> 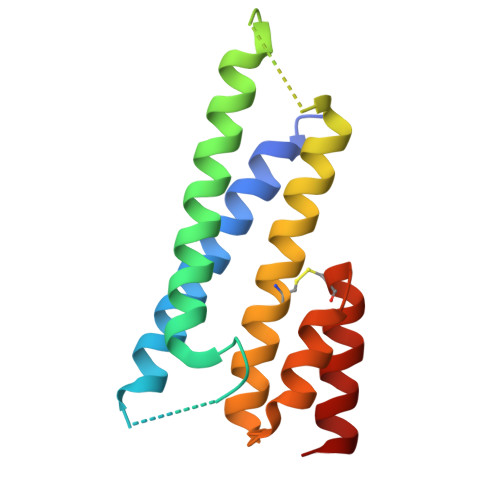GSHMSTEQIQKRTAAIQKRIAAIQKRIYAMTASGGAGAAGAGAGMSIEEITKQIAAIQLRIVGDQVQIAYQTASGAGAGAGGMSTEEIQKQIAAIETQICKIEAAIELKEAGITSDFYFELINKAKTCEGVEALKEHILAAHT> GPLSFSLGLQDFDLLRVIGRGSYAKVLLVRLKKTDRIYAMKVVKKELVNDDEDIDWVQTEKHVFEQASNHPFLVGLHSCFQTESRLFFVIEYVNGGDLMF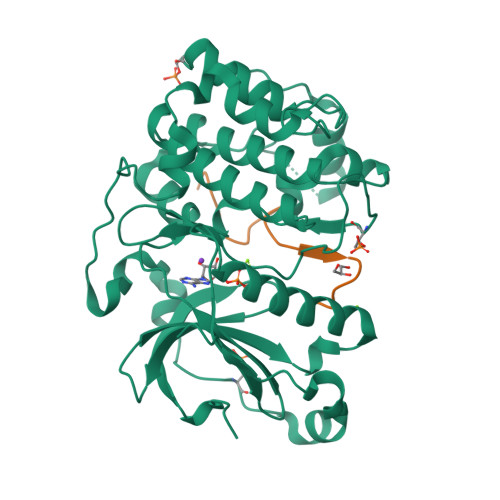HMQRQRKLPEEHARFYSAEISLALNYLHERGIIYRDLKLDNVLLDSEGHIKLTDYGMCKEGLRPGDTTSTFCGTPNYIAPEILRGEDYGFSVDWWALGVLMFEMMAGRSPFDIVGSSDNPDQNTEDYLFQVILEKQIRIPRSLSVKAASVLKSFLNKDPKERLGCHPQTGFADIQGHPFFRNVDWDMMEQKQVVPPFKPNISGEFGLDNFDSQFTNEPVQLTPDDDDIVRKIDQSEFEGFEYINPLLMSAEECV;> LAFQREGFGRQSMSEKRTKQ> MNRFGTAQVNLNFDKNFSLKESSLDWLAPWYDSASFLFFSQLGIRNKDSRNTLNLGVGIRTLENGWLYGLNTFYDNDLTGHNHRIGLGAEAWTDYLQLAANGYFRLNGWHSSRDFSDYKERPA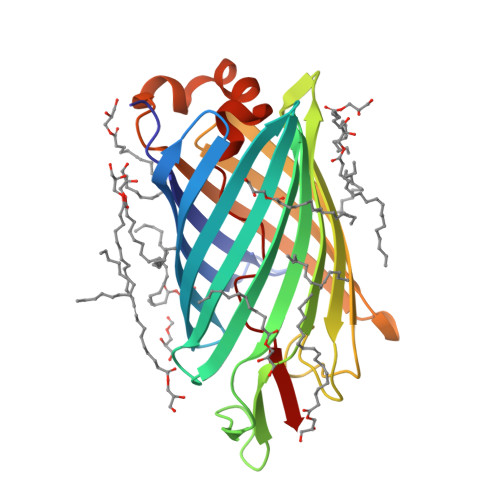TGGDLRANAYLPALPQLGGKLMYEQYTGERVALFGKDNLQRNPYAVTAGINYTPVPLLTVGVDQRMGKSSKHETQWNLQMNYRFGESFQSQLSPSAVAGTRLLAESRYNLVDRNNNIVLEYQ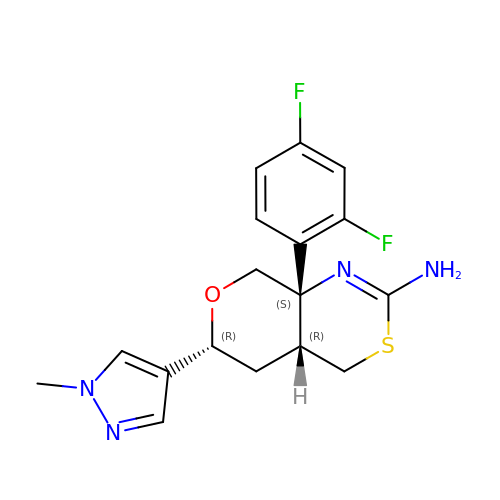(4aR,6R,8aS)-8a-(2,4-difluorophenyl)-6-(1-methyl-1H-pyrazol-4-yl)-4,4a,5,6,8,8a-hexahydropyrano[3,4-d][1,3]thiazin-2-amine | C17 H18 F2 N4 O S | JYDYMWJEZLKIBS-CXMBCZLWSA-N>MSPIPLPVTDTDDAWRARIAAHRADKDEFLATHDQSPIPPADRGAFDGLRYFDIDASFRVAARYQPARDPEAVELETTRGPPAEYTRAAVLGFDLGDSHHTLTAFRVEGESSLFVPFTDETTDDGRTYEHGRYLDVDPAGADGGDEVAL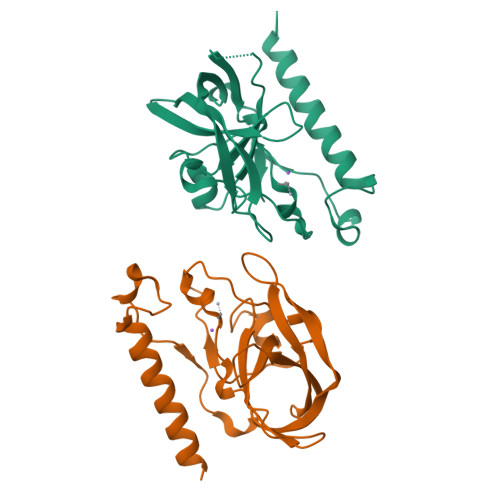DFNLAYNPFCAYGGSFSCALPPADNHVPAAITAGERVDADLEHHHHHH[2x]> YAPSALVLTVGKGVSATTAAPERAVTLTCAPGPSGTHPAAGSACADLAAVGGDLNALTRGEDVMCPMVYDPVLLTV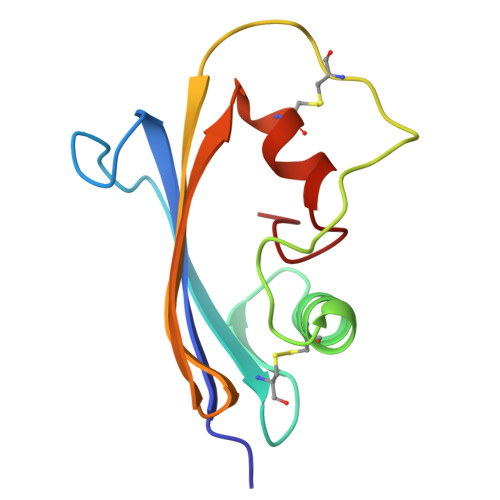DGVWQGKRVSYERVFSNECEMNAHGSSVFAF> VEATAQETDRPRFSFSIAAREGKARTGTIEMKRGV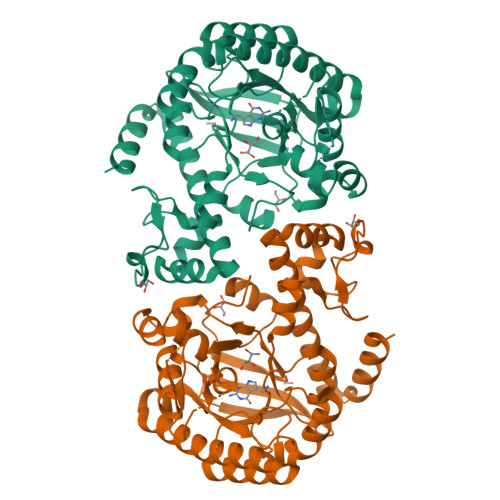IRTPAFMPVGTAATVKALKPETVRATGADIILGNTYHLMLRPGAERIAKLGGLHSFMGWDRPILTDSGGFQVMSLSSLTKQSEEGVTFKSHLDGSRHMLSPERSIEIQHLLGSDIVMAFDEVTPYPATPSRAASSMERSMRWAKRSRDAFDSRKEQAENAALFGIQQGSVFENLRQQSADALAEIGFDGYAVGGLSGGEGQDEMFRVLDFSVPMLPDDKPHYLMGVGKPDDIVGAVERGIDMFDCVLPTRSGRNGQAFTWDGPINIRNARFSEDLKPLDSECHCAVCQKWSRAYIHHLIRAGEILGAMLMTEHNIAFYQQLMQKIRDSISEGRFSQFAQDFRARYFARNS Angiogenin (ANG), a 14-kDa basic protein is an angiogenic ribonuclease and member of the bovine pancreatic ribonuclease (RNase A) family (also known as RNase 5). Like RNase A, ANG cleaves preferentially on the 3′ side of pyrimidines and follows a transphosphorylation/hydrolysis mechanism. In addition, the crystal structure of human ANG has revealed that it has an RNase A fold and the catalytic triad (residues H13, K40 and H114) is conserved. The enzymatic activity of ANG is several orders of magnitude lower than that of RNase A towards conventional RNase substrates, but essential for its angiogenic effect.

ANG residues 60–68 are part of an external region that includes strand B2 and loops on either side. Based on known experimental data to date this region has been predicted to form part of the cell receptor binding site44. K60 forms part of this region at one end of the segment and is located on the surface of the molecule in the 3D structure. Mutation of the residue to Glu retains ~80% of the enzymatic activity. Previously it has been shown that chemical modification of K60 retained 34% activity and this surface residue has minor catalytic role. In the K60E PD variant structure the mutated residue gains a new interaction with E58, which seems to result in a level of repulsion of neighbouring residues in comparison to the wild-type ANG structure.

> MQDNSRYTHFLTQHYDAKPQGRDDRYCESIMRRRGLTSPCKDINTFIHGNKRSIKAICENENGNPHRENLRISKSSFQVTTCKLHGGSPWPPCQYRATAGFRNVVVACENGLPVHLDQSIFRRP>[2x]GSMAELEHLAQNISKSHLETCQYLREELQQITWQTFLQEEIENYQNKQREVMWQLCAIKITEAIQYVVEFAKRIDGFMELCQNDQIVLLKAGSLEVVFIRMCRAFDSQNNTVYFDGKYASPDVF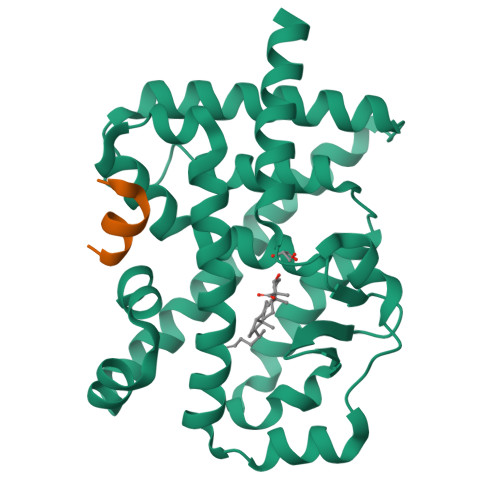KSLGCEDFISFVFEFGKSLCSMHLTEDEIALFSAFVLMSADRSWLQEKVKIEKLQQKIQLALQHVLQKNHREDGILTKLICKVSTLRALCGRHTEKLMAFKAIYPDIVRLHFPPLYKELFTSEFEPAMQIDG;>[2x]TLLQLLLGHKNE>XGELKAIAQELKAIAKELKAIAWEA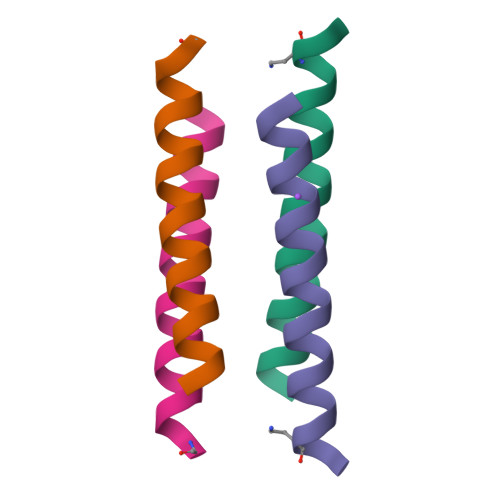KAIAQGX[2x]(2E,4E)-11-METHOXY-3,7,11-TRIMETHYLDODECA-2,4-DIENOIC ACID | C16 H28 O3 | 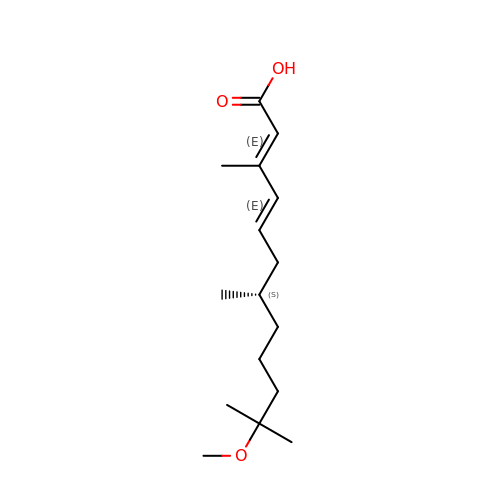MNYBEULOKRVZKY-ATCPXPEISA-N>[2x]XTYKITVRVYQTNPNAFF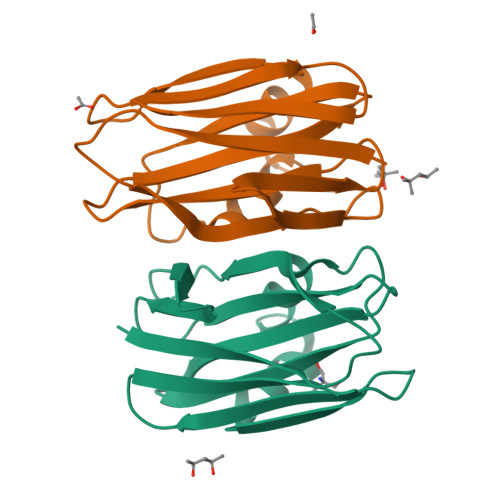HPVEKTVWKYANGGTWTITDDQHVLTMGGSGTSGTLRFHADNGESFTATFGVHNYKRWCDIVTNLAADETGMVINQQYYSQKNREEARERQLSNYEVKNAKGRNFEIVYTEAEGNDLHANLIIG>[2x]IRYPNGKTFQPKHSVSSQNSQKRAPSYSNRGMTLEDDLNETNKYYLTNQIAVIHKKPTPVQIVNVHYPKRSA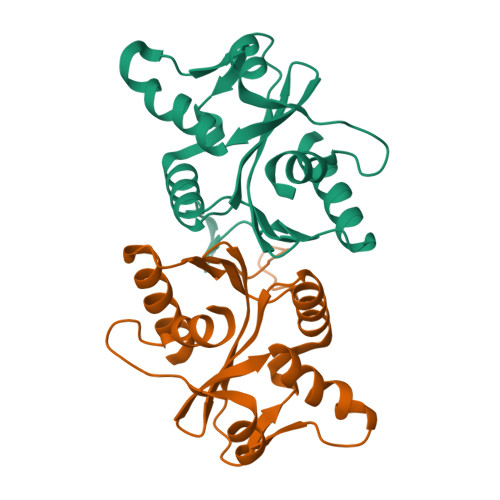AVIKEAYFKQSSTTDYNGIYKGRYIDFEAKETKNKTSFPLQNFHDHQIEHMKQVKAQDGICFVIISAFDQVYFLEADKLFYFWDRKEKNGRKSIRKDELEETAYPISLGYAPRIDYISIIEQLYFSPSSGAKG>[4x]MGHHHHHHAENLYFQGADPFESYNPEFFLYDIFLKFCLKYIDGEICHDLFLLLGKYNILPYDTSNDSIYACTNIKHLDFINPFGVAAGFDKNGVCIDSILKLGFSFIEIGTITPRGQTGNAKPRIFRDVESRSIINSCGFNNMGCDKVTENLILFRKRQEEDKLLSKHIVGVSI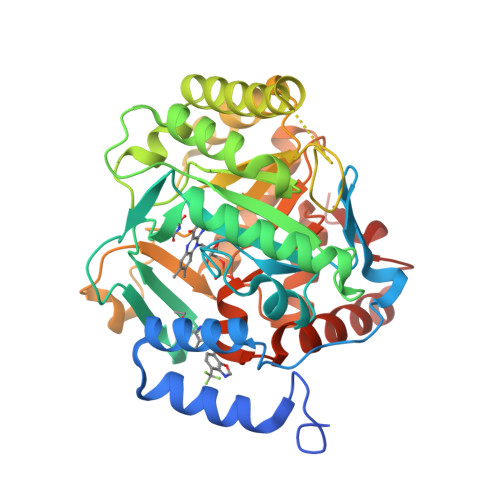GKNKDTVNIVDDLKYCINKIGRYADYIAINVSSPNTPGLRDNQEAGKLKNIILSVKEEIDNLEKNNIMNDEFLWFNTTKKKPLVFVKLAPDLNQEQKKEIADVLLETNIDGMIISNTTTQINDIKSFENKKGGVSGAKLKDISTKFICEMYNYTNKQIPIIASGGIFSGLDALEKIEAGASVCQLYSCLVFNGMKSAVQIKRELNHLLYQRGYYNLKEAIGRKHSKS>[2x]MSSIA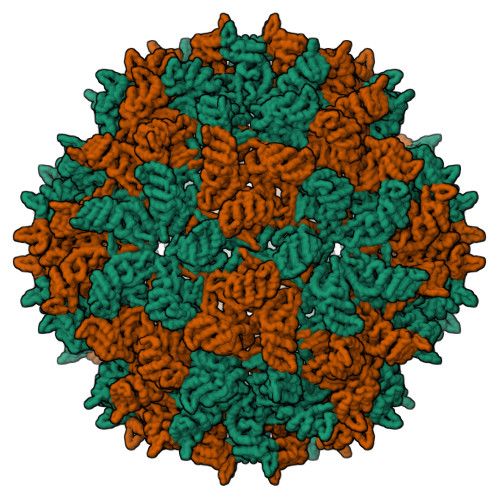PTDSVSSSGKRSKPGKRERQQARSAVGSAGGKPASASKAAAFAQGGSSDPVPMPGKYPVVFSTGAGEPTRDQEFALPVHKAFPLFGSVSDKYRRNPRYAEFRAHSEFTDGVFGTHLAVSSLLRLAQQLVHAHVNMGLPLGDFAPLASSDVRIPSALASVVNQFGEFSSPSIGTRFLLRDFEHAVSRVVFLADQLWTNGNSHHIFARSWLPMSNNDGNFKTIVASRLLEFISAGDLSILPTVLEDAVLSGEVPEAWEQVKDLLGDAPGVGQVDRRDRFDFLFKSYADVGQFTTAFTTQAASDVLTELGLPWNSPSAGHLNWQYSTKQRFTFLADTWAKLSAAYSQFFELSSGLATRQSATGSHAQMVDLTSVEGVTVLKAALALSAPEFSLAACFPPSCIFVGGLTRRVVVTTSLSVSQRATEFCQMDWR>[2x]MSLSLPLFYAPDIEQSDRLPDDEAGHILRVLRMQAGDRLRLTDGRGSFFDAVIETADRKSCYVSVCGQESWQKPWRDRITIAIAPTKQSERMEWMLEKLVEIGVDEVVFIESEHSERRRIKAERLERIAISAMKQSLKASFPVI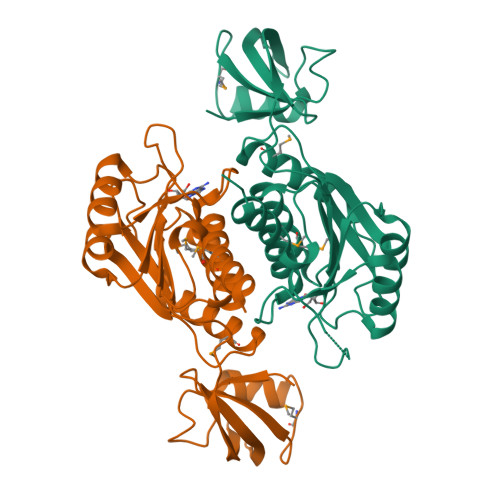RVNIPIQTVIADTPKAAVRLIAYVDEAVRAEITQGRGYPSDFYHVGQDVLILIGPEGDFSPSEVESALLAGFAPVSLGESRLRTETAGLVACQWIHTLQACYRIGEGHHHHHH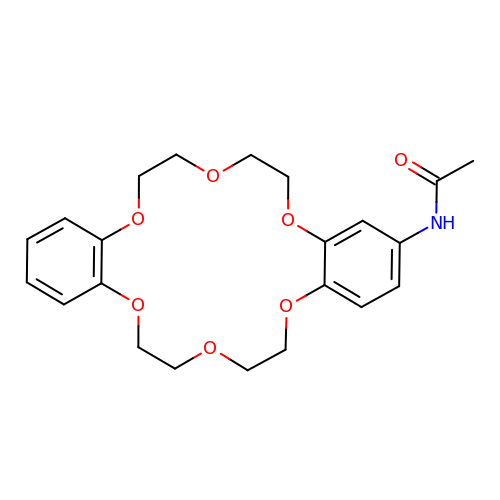N-(6,7,9,10,17,18,20,21-octahydrodibenzo[b,k][1,4,7,10,13,16]hexaoxacyclooctadecin-2-yl)acetamide | C22 H27 N O7 | YHKGWOJTUMJPNW-UHFFFAOYSA-N>[4x]MKLWIDTDCGIDDATAILICLANPSIEIVGISCIGGNASLQNVIRNVNRTLKVWGKTDIPIFGGCQAPLVQPKMEIPHIHGGDGLGDINDNDFGTNTPNKLEKEHAVNALIHAANTIEDLNILCLAPLTNIAIALSMAPEAILKIKHFYIMGG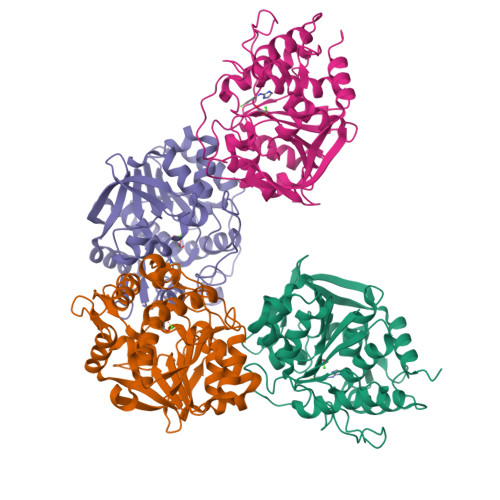AENGKGNITPYGEFNWRADPEAAQIVLQTYPQYQTTIASWTLAVFNSFNANDYDFFNLDGNLVRRFIRETWKPIIAFDGGRICPADPLAAFIAVYGDRAIKRAERLHLSMVLEGEKLGMSLAEPDEKGCLVVKECDAELFVKILRELQDHQ> PCVVGGQADTIYPAIANQMAHQMHEDAQTEASKRGLAKLRADAKQGIYKKNRKPQELSNICNITLQHSNDSRNGNNGGACTGKDGNNERFKIGTEWKIGEKVETTDTDAYIPPRRQHMCTSNLENLNVSWVTEDGKAIHSLLGDVQLAAKMDADEIIKRYKKHNTLTDPIQQKDQESICRAVRYSFADLGDIIRGRDLWEHGDQTKLQGHLQIIFGKIKEEIKKKHPGINGNDKYKGDEKNNPPYKQLREDWWEANRHQVWRAMQCELKNLKKSNGDCHYNSRGTPLDDYIPQRLRWMVEWAEWFCKMQSQEYDKLMKQCSQCMSKGGDCRKGDVNCTSCEQACEEYKKKIKKWEKQWNKIKDKYEELYLQAKIAFAGTSFGGGDRDYQQMVHFFKELQKVTGDTTLGDTTSPYSTAAGYIHQEGHVDECTEQTQFCKNRNGNTASGKEDDNYTFKDPPPKYANACKCD

However, the parasite also displays members of variant protein families on the surface of infected erythrocytes, including the multidomain Plasmodium falciparum erythrocyte membrane proteins 1 (PfEMP1). These PfEMP1 cause infected erythrocytes to adhere to the surfaces of blood vessels and tissues, removing them from circulation and protecting the parasite within from spleen-mediated destruction. ICAM-1 binding is mediated by a subset of Duffy binding-like (DBL) domains, the DBLβ domains, which are found in either A-type or BC-type PfEMP1 (26–29). To understand how these BC-type PfEMP1 interact with ICAM-1, we have determined the structure of the DBLβ domain of the B-type IT4var13 PfEMP1 in complex with the N-terminal domains of ICAM-1, revealing divergent, but similar, modes of ICAM-1 binding across the PfEMP1.

The DBLβ domain from IT4var13 formed crystals which diffracted to 2.17 Å resolution. The IT4var13 DBLβ domain adopts the classical DBL domain fold, consisting of an α-helical core decorated by extensive loops. Comparison of the unbound and the ICAM-1D1D2-bound DBLβ domains showed little variation in structure upon ligand binding (root mean square [rms] deviation of 1.07 Å over backbone Cα), with variation predominantly located in loops (residues 805 to 809, 833 to 840, and 1107 to 1117). Secondly, a loop from the DBLβ domain (residues 1107 to 1117) interacts through backbone–backbone hydrogen bonds with ICAM-1D1 to add an antiparallel β-strand to the A′GFC β-sheet of ICAM-1D1. In the unbound DBLβ domain, this loop adopts a different conformation which is stabilized through crystal contacts, indicating that it is flexible and becomes stabilized upon interaction with ICAM-1. This is analogous to a different intrinsically disordered loop that becomes ordered to form part of the ICAM-1 binding site of A-type PfEMP1 (22).>[6x]MKTIFSGIQPSGVITIGNYIGALRQFVELQHEYNCYFCIVDQHAITVWQDPHELRQNIRRLAALYLAVGIDPTQATLFIQSEVPAHAQAAWMLQCIVYIGELERMTQFKEKSAGAAAAAAGLLTYPPLMAADILLYNTDIVPVGEDQKQHIELTRDLAERFNKRYGELFTIPEARIPKVGARIMSLVDPTKKMSK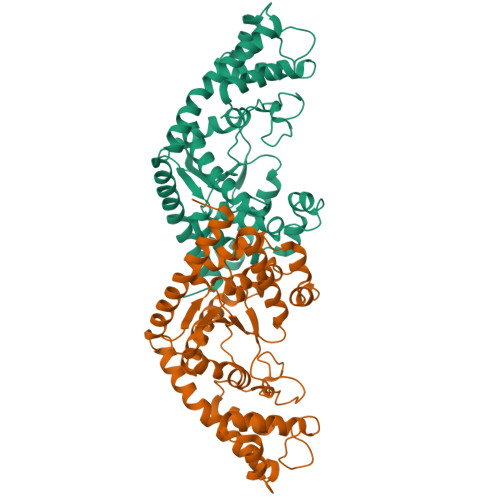SDPNPKAYITLLDDAKTIEKKIKSAVTDSEGTIRYDKEAKPGISNLLNIYSTLSGQSIEELERQYEGKGYGVFKADLAQVVIETLRPIQERYHHWMESEELDRVLDEGAEKANRVASEMVRKMEQAMGLGR> GMSVNGIEVAKPFIAATVNVLSTMAGIQPQPGKPYVKKNNVAKGDVSAVIGITGHKNGSISVTFTKSCAIALVKGMLGDDIQDILQDTKDAVGEVTNMISGQARAGLAEMGMVFQGSTPSVIMGDGHTISHVTK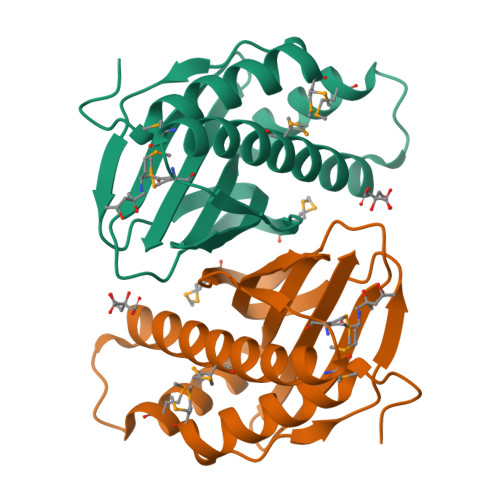SPIMAIPFLTNHGEFTVEFCFE> MSMAEMLRRDEGLRLKVYWDTEGYPTIGIGHLIMKQPVRDMAQINKVLSKQVGREITGNPGSITMEEATTLFERDLADMQRDIKSHSKVGPVWQAVNRSRQMALENMAFQMGVGGVAKFNTM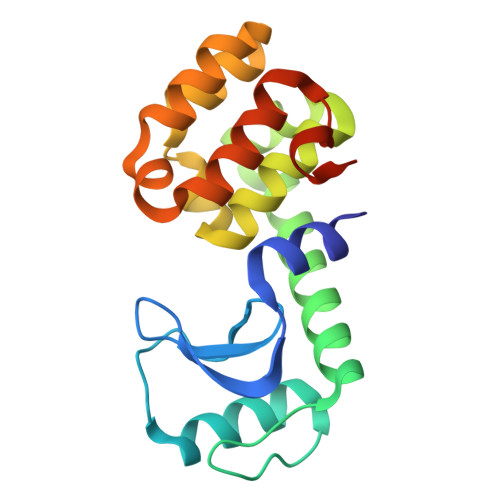LTAMLAGDWEKAYKAGRDSLWYQQTKGRASRVTMIILTGNLESYGVELEHHHHHH> MRRGSGFVHLNTPAAISYSPGQQVSLSDLRQKRRREECVVLPPIMTVWRSAFSQYTKMWGLTKFAGDIEAEREGEGPILPPIREETVVKSTTHSFKGKSTTVAAAVATPPGEKGIEIVSHHKLCGKQRFVYPDHDGVLSSGIVPKVVISKEEEEEMEANKKYYISPQEMTEEERNAFEELDAMWKSYARGRSEQ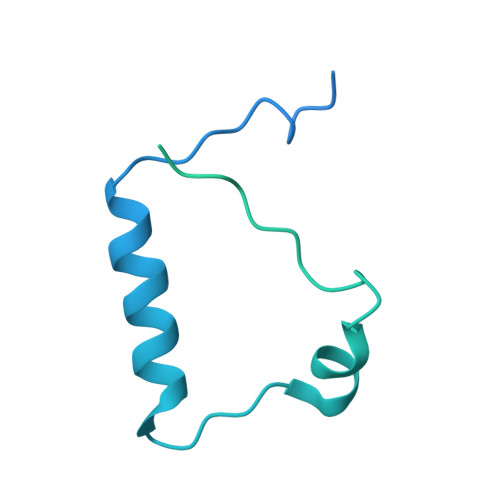GARHRAFAGTVTPGDAMTEVEEETGNNRGNARRRLESHTPRQHPQESAAEGNSVAHNTEEALDDALRLIDELLEFN1-[(3aR,7aR)-1-(7H-pyrrolo[2,3-d]pyrimidin-4-yl)octahydro-6H-pyrrolo[2,3-c]pyridin-6-yl]propan-1-one 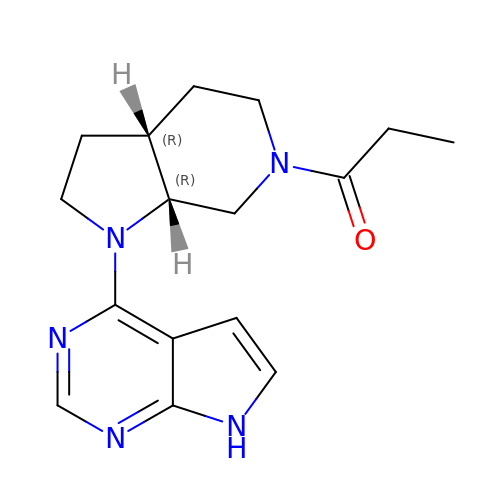| C16 H21 N5 O | ZXWSRKWKYQKIOB-AAEUAGOBSA-N> MAVKITMTSGGVGKELEVLKKQLEMFHQQYPDIEVEIIPMPDSSTERHDLYVTYFAAGETDPDVLMLDVIWPAEFAPFLEDLTADKDYFELGEFLPGTVMSVTVNGRIVAVPWFTDAGLLYYRKDLLEKYGYDHAPRTWDELVEMAKKISQAEGIHGFVWQGARYEGLVCDFLEYLWSFGGDVLDESGKVVIDSPEAVAALQFMVDLIYKHKVTPEGVTTYMEEDARRIFQNGEAVFMRNWPYAWSLVNSDESPIKGKVGVAPLPMGPGGRRAATLGGWVLGINKFSSPEEKEAAKKLIKFLTSYDQQLYKAINAGQNPTRKAVYKDPKLKEAAPFMVELLGVFINALPRPRVANYTEVSDVIQRYVHAALTRQTTSEDAIKNIAKELKFLLGQHHHH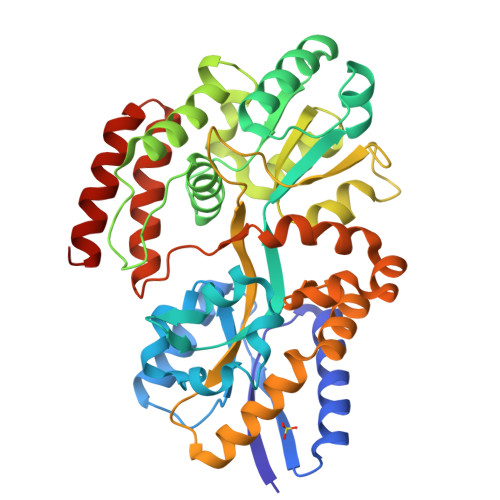HH>[3x]MCI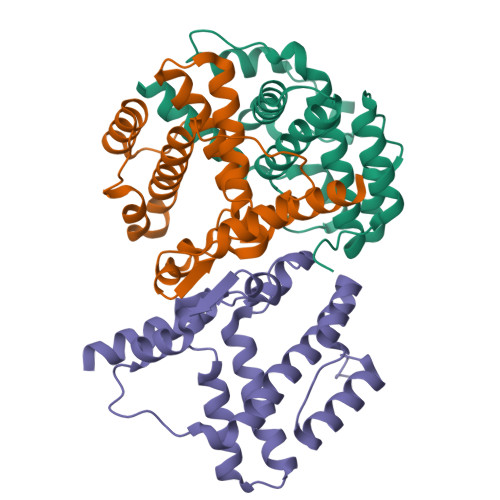IKPMDDVVKFIHEVGSLKLTPRSGWLKLGIRLPESVAEHNFRAAIIAFILALKSGESVEKACKAATAALFHDLHEARTMDLHKIARRYVSCDEEGAREEQLSWMESKPDFSDVEVYVSDADKLELAFQGVEYSQQVSYAIRFAENVELKTDAAKEIYRVLMERKNPVWWR(5S)-5-[(1R)-1-(1H-indol-3-yl)ethyl]-2-(methylamino)-1,3-oxazol-4(5H)-one 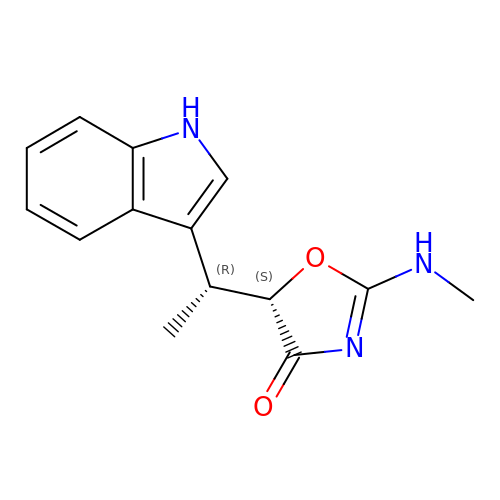| C14 H15 N3 O2 | GNTVWGDQPXCYBV-PELKAZGASA-N>[9x]GVQPLATQCFQLSNMFNPQTEEEVGWDTEIKDDVIEECNKHGGVIHIYVDKYSAQGNVYVKCPSIAAAIAAVNALHGRWFAGKMITAAYVP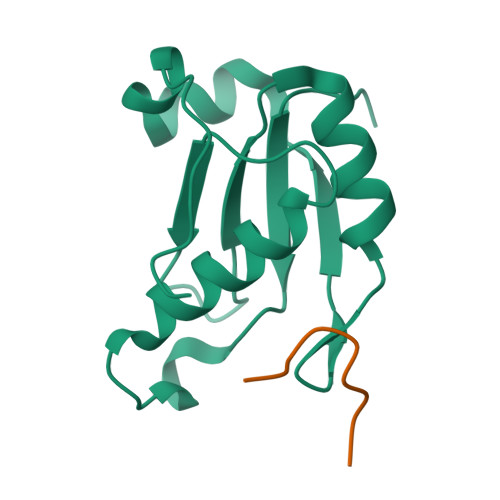LPTYHNLFPDSMTATQLLVPSRR;>GKKKVRKYWDVPPPGFEHITPMQYKAMQA[9x]> GPGSMVTQPEAVDRLDPLLRAVATARIDFTAESILTIRE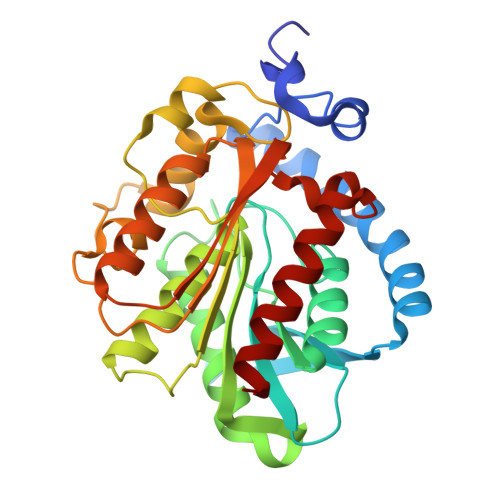SMNQRRREAAATETAAAGVAVADDVVTGEAGRPVPVRIYRAAPTPAPVVVYCHAGGFALGNLDTDHRQCLELARRARCAVVSVDYRLAPEHPYPAALHDAIEVLTWVVGNATRLGFDARRLAVAGSSAGATLAAGLAHGAADGSLPPVIFQLLHQPVLDDRPTASRSEFRATPAFDGEAASLMWRHYLAGQTPSPESVPGRRGQLAGLPATLITCGEIDPFRDEVLDYAQRLLGAGVSTELHIFPRACHGFDSLLPEWTTSQRLFAMQGHALADAFYP>[3x]MASEPDRLDQIDFPVRTVTVVVPFAKGGPTDTVARLITAEMAKTLGQPIEIENMLGA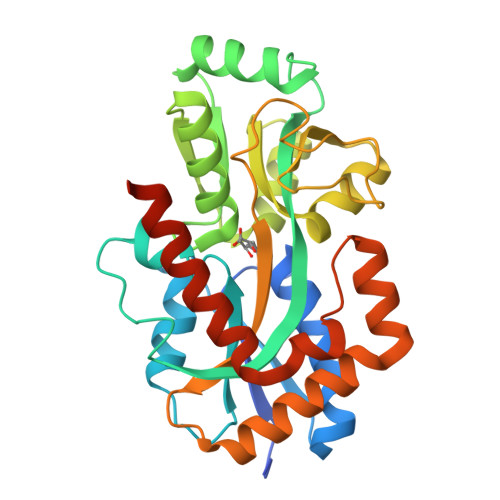GGTLAATRVAHAAPDGHTLIVGHLGTHGAAVALFPKLAYRPDKDFTPVALLTEMPVLLLARKQFPPKDLSEFASYVESHTDNLNVAHAGFGSVSYASCLLLNRLLKVDPTGVPFSGTGPALQALVEGQVDYMCDQIVNAVPALREGKVKAYVIAASERDPVVPDVPTAREAGLPGFQVGAWTGLFAPRGTPEPIVAKLNAAVSRALDQSDVRTRLTDLGALVPRPEQRAPVVLAQLVQEEISRWEDVVEGTTPLEHHHHHH>[4x]GAMGMHGRRLGVMGGTFDPIHYGHLVAASEVADLFDLDEVVFVPSGQPWQKGRQVSAAEHRYLMTVIATASNPRF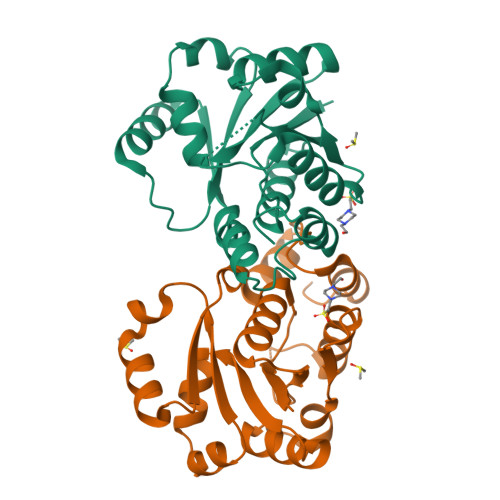SVSRVDIDRGGPTYTKDTLADLHALHPDSELYFTTGADALASIMSAQGWEELFELARFVGVSRPGYELRNEHITSLLGQLAKDALTLVEIPALAISSTDCRQRAEQSRPLWYLMPDGVVQYVSKCRLYCGACDAGARSTTSLAAGNGL>MAHHHHHHMNRVLYPGTFDPITKGHGDLIERASRLFDHVIIAVAASPKKNPLFSLEQRVALAQEVTKHLPNVEVVGFSTLLAHFVKEQKANVFLRGLRAVSDFEYEFQLANMNRQLAPDVESMFLTPSEKYSFISSTLVREIAALGGDI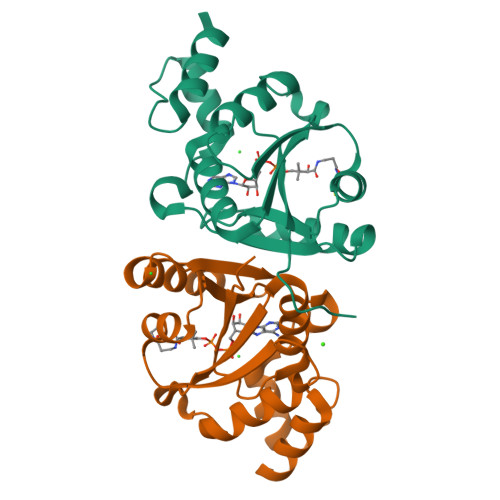SKFVHPAVADALAERFKR[6x]>MGLCLAKRNHDADDDEPHIELAGGNVHLITTKERWDQKLSEASR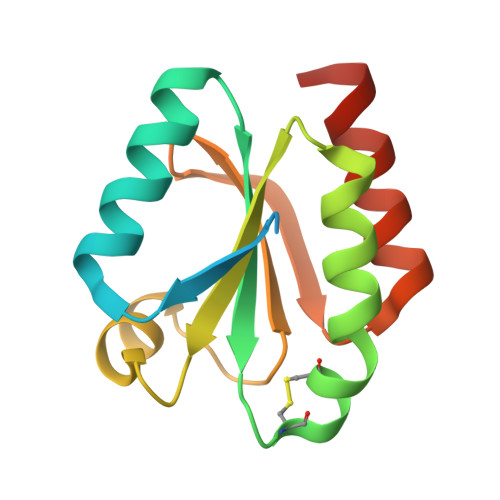DGKIVLANFSARWCGPCKQIAPYYIELSENYPSLMFLVIDVDELSDFSASWEIKATPTFFFLRDGQQVDKLVGANKPELHKKITAILDSLPPSDK[2x]>[2x]MARCDVLVSADWAESNLHAPKVVFVEVDEDTSAYDRDHIAGAIKLDWRTDLQ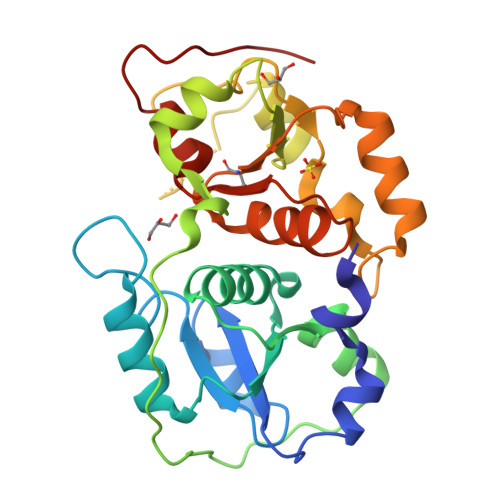DPVKRDFVDAQQFSKLLSERGIANEDTVILYGGNNNWFAAYAYWYFKLYGHEKVKLLDGGRKKWELDGRPLSSDPVSRPVTSYTASPPDNTIRAFRDEVLAAINVKNLIDVRSPDEFSGKILAPAHLPQEQSQRPGHIPGAINVPWSRAANEDGTFKSDEELAKLYADAGLDNSKETIAYCRIGERSSHTWFVLRELLGHQNVKNYDGSWTEYGSLVGAPIELGS Here, we take a structural approach to assess the relatedness of these eukaryotic-like proteins in Asgard archaea, the closest known prokaryotic relatives to eukaryotes. Asgard archaea roadblock, longin and TRAPPC3 domain-containing proteins form dimers similar to those found in the eukaryotic TRAPP and Ragulator complexes. Here, we adopted an X-ray crystallography approach to compare the structures of a potential Asgard Rab small GTPase, several RBs and two TRAPPC3 proteins to their eukaryotic counterparts, with a focus on Thor and MKD1. We conclude that the emergence of these protein architectures predated eukaryogenesis, however further adaptations occurred in proto-eukaryotes to allow these proteins to regulate distinct internal membranes.

Finally, we investigated the TRAPPC3-like proteins from Thor. The crystals were pink in color indicating potential Zn2+ binding. We scanned Zn2+ fluorescence for AB25 Thor-TRAPPC3 using X-rays to confirm the identity of the cation and collected multiple anomalous dispersion (MAD) diffraction data around the Zn2+ edge to solve the structure at 1.91 Å. We further analyzed the homology around the Thor-TRAPPC3 Zn2+-binding site. We found that the predicted Zn2+-binding sites and the experimentally determined sites are not completely conserved in positions of the coordinating residues, rather they appear in similar regions and appear to serve the same function in tethering the β-sheet to the D α-helix to create cavities. Interestingly, mouse TRAPPC3 has evolved to replace the Zn2+-binding site by a hydrogen bond. We speculate that Thor-TRAPPC3 may also bind small molecules, potentially being involved in ligand transport. The cavities appear to be accessible from the exterior close to the dimerization interfaces. Furthermore, we uncover structural evidence that TRAPPC3-like proteins exist in several branches of Asgard archaea and are likely to share a common ancestor gene with the V4R-like domain.

>[2x]GPMPKIENPLLISLYSYYVEKTLSETKSIEEANQRLRELGKEIGQQVYLNTEIVEKTKDNVATREDVAKLIEIIYKVLFDKKPNDIDMKSARGSVRITDDDCVWCQEVNLEGMRGFGYCEVFSGILEAVLEFKDVDAKVFQEMSKATGADSCIWNVRLV> GLPVMN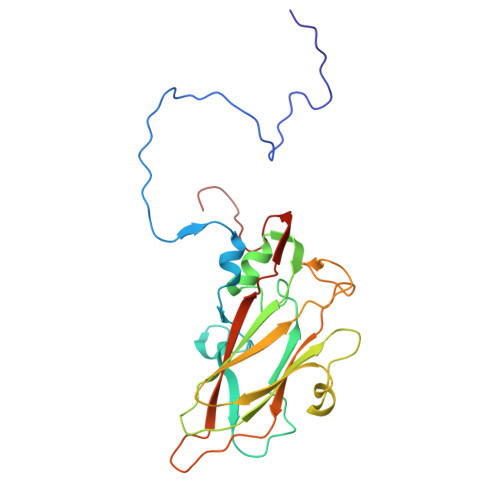TPGSNQFLTSDDFQSPSAMPQFDVTPELNIPGEVQNLMEIAEVDSVVPVNNVEGKLDTMEIYRIPVQSGNHQSSQVFGFQVQPGLDNVFKHTLLGEILNYYAHWSGSIKLTFVFCGSAMATGKFLLAYAPPGANAPKSRKDAMLGTHIIWDVGLQSSCVLCIPWISQTHYRLVQQDEYTSAGNVTCWYQTGIVVPAGTPTSCSIMCFVSACNDFSVRLLKDTPFIEQSALLQ trihydroxy{(1S)-1-[(methylsulfonyl)amino]ethyl}borate(1-) | C3 H11 B N O5 S | 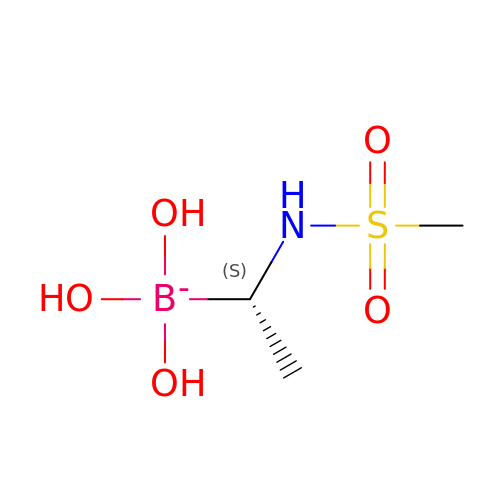ZTYRBLZCLIYDCR-GSVOUGTGSA-N>[8x]MVKNWLFGKKRKEDADALATLKGQQNRLQAEARNLERQSDEQKILASKMLKAGNKAGARQALKRRAVFMKRLNTVHNTAMNLQAQIDSIQTATSTAETVKAMELGTKVVGEKIKTVSPERTERVMDSVMEQRDQIEMMTEALSDPSLSEGILDFEDDAAIDEQLAQLEAEMDLGTTTSLPDVSGLPSTPVGTGEKEEDTSELEAELEGLKKKMSEDKQ

To aid these processes, cells from across the tree of life use a conserved family of polymer-forming endosomal sorting complex required for transport III (ESCRT-III) proteins that deform, cut, and repair membranes (1–3). Individual ESCRT-III proteins are small and have a simple set of α helices (α1 to α5) that define the functional core of the protein. The most stripped-down version of the ESCRT-III system is found in Asgard archaea, the closest prokaryotic relatives of eukaryotes, which have as few as two ESCRT-III homologs. We show that Asgard ESCRT-IIIB assembles into parallel arrays on planar membranes to initiate membrane deformation, from where it recruits ESCRT-IIIA to generate composite polymers.

The structure of membrane-bound Asgard ESCRT-IIIB also revealed that the protein binds membranes via the N terminus of α1 and the loop connecting helices α3 and α4. This interface includes an exposed region of continuous positive charge as well as hydrophobic residues, consistent with the binding of filaments to negatively charged membranes. By superimposing our high-resolution structure onto the membrane-bound map, we noticed that hydrophobic residues of helix α1 were positioned to insert into the lipid core of the membrane. While this interface differs from the reported interaction site of CHMP1B (A-type) with membranes, it is similar to the membrane binding interface of Snf7 (B-type) and CHMP2A-CHMP3 (A-type). An analysis of adjacent membrane-bound protofilaments revealed that interactions between them are mediated by their planar faces through the positive charges of helix α1 and negative charges of α4. A comparison with our off-membrane structure revealed a slightly smaller intersubunit distance in the membrane-bound protofilament (~3 nm versus 2.7 nm, respectively). This was accompanied by a change in the angle between helices α3 and α4 (off-membrane: 145°; on-membrane: 116°). The conformational differences between the membrane-bound and unbound polymers may be influenced by the distinct interactions therein, underscoring the adaptability of the ESCRT-IIIB protofilament. We show how protofilaments are able to adapt to different membrane curvatures, likely through the intrinsic flexibility of ESCRT-IIIB at the hinge between helices α3 and α4.In this work, we describe the AKR from the termite C. gestroi (CgAKR-1), a founding member of a new AKR subfamily of potential biotechnological interest. CgAKR-1 displayed major structural differences compared with others AKRs, including the differences in the amino acid composition of the substrate-binding site, providing basis for classification as a founding member of a new AKR subfamily (family AKR1 I). The most related and well-characterized family members in this database are human AKR (AKR1A1) and nematode AKR from Caenorhabditis elegans (AKR1G1). Generally, members of the AKR1 family have broad specificity for aldehydes, are cytosolic and monomeric proteins, and interact strongly with NADPH as a cofactor. Thus, we concluded that in addition to its ability to reduce aldehydes, CgAKR-1 had an NADPH oxidase-like function and could generate ROS, such as H2O2, during in vitro assays.

The three-dimensional structure of CgAKR-1 revealed a conserved structure, known as the (β/α)8 barrel, within the AKR superfamily. This structure consisted of eight β-strands in the central region surrounded by eight α-helices. The NADP-binding site is buried in the protein structure and is highly conserved throughout members of the AKR superfamily, despite the low similarity of other regions of the protein. CgAKR-1 displays structural determinants that underlie the preference for NADPH, which is related to the positively charged arginine residues that bind to pyrophosphate backbone and the 5′ phosphate group of NADPH. The amino acids W24, N47, Y52, H114, S166, N167, Y214, I217, S219, K276, S277, R282, E285, and N286 surrounded the cofactor. In addition, the catalytic residues were identified as D47, Y52, K81, and H114 and were also conserved. The superposition of CgAKR-1 chain A with AKRs complexed with substrates indicated that the substrate-binding site was delimited by the amino acids W24, M51, Y52, H114, L115, W128, R229, F314, and M316. One major feature of the CgAKR-1 structure was the presence of a longer loop (known as loop B) between the seventh and eighth β-strands of the barrel (residues L222 to L242) compared with that of other AKRs. This longer loop also exhibited high mobility based on high B-factor in chain A, which could not be modeled in chain B owing to the absence of a defined electron density. Consequently, the unparalleled long loop B from CgAKR-1 seemed to play an important role, not only in cofactor binding but also in substrate interaction owing to the arginine (R229) positioned towards the substrate-binding site.

>[2x]GSHMASMPKQLSSVTFHNGRKMPVVGLGTWQSPPEEVTAAIDVALEVGYRHIDTAFMYQNEAAIGKTLKKWFDSGKLKREDVFIVTKLPPIGNRAESVEKFLTKSLEALQLDYVDLYLIHLPVGFQYKGDDNLWPRGEAGEFLIDTSTDLISLWKAMEAQVDAGRTRSVGLSNFNSRQIARIVKSARIRPANLQVELNVYFQQRELVAFCRALDITVCAYAPIGSPGLANVIKARGAEVPESAKFDPLTDPVVLKIAEHHKKTPAQVLLRHCMQRDIVVIPKSTNAGRIKENFQVFDFELSKAEVDELDSLDKRAAGRRFRMDQYKGLREHPEHPYDEPY>[3x]C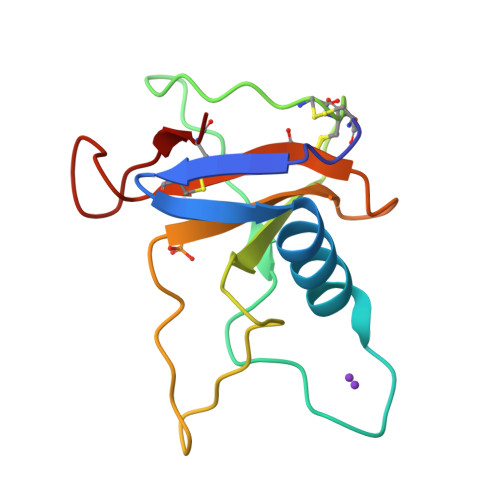DIPQSTNCGGNVYSNDDINTAIQGALDDVADGDRPDNYPHQYYDEASEDITLCCGSGPWSEFPLVYNGPYYSSRDNYVSPGPDRVIYQTNTGEFCATVTHTGAASYDGFTQCS> MKKNAKQIVHELYNDISISKDPKYSDILEVMQKVYLKLEKQKYELDPSPLINRLVN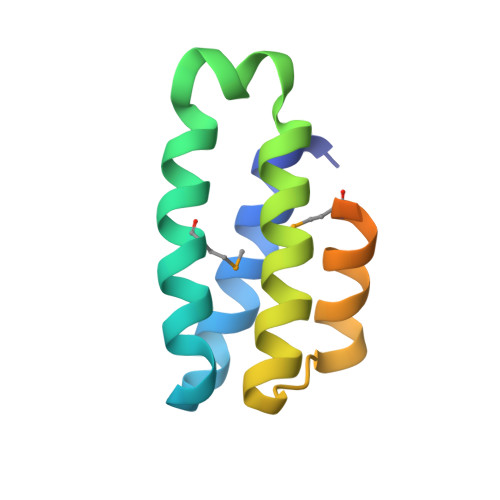YLYFTAYTNKIRFTEYQEELIRNMSEIGRTAGINGLYRADYGDKSQF2-(4-acetylphenyl)-4-methyl-1H-isoindole-1,3(2H)-dione 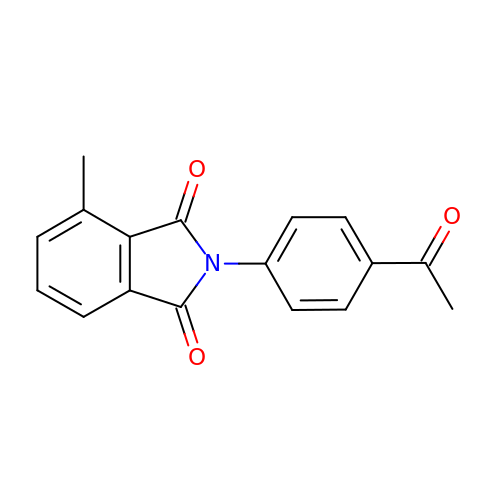| C17 H13 N O3 | RQFQRVRMHYMTAU-UHFFFAOYSA-N Unphosphorylated STATs form an anti-parallel dimer/monomer equilibrium, and upon efficient recruitment to the cognate receptor–kinase complex, are phosphorylated on a specific tyrosine residue, which promotes parallel dimerization by conformational rearrangement. The activated STAT dimer translocates to the nucleus, initiating transcription of target genes and altering chromatin involved in loop formation in enhancer-promoter landscapes. The canonical domains of the STAT family are all present with the coiled-coil domain (CCD, S138-T331), DNA-binding domain (DBD, F332-V470), linker domain (H471-D591), and SH2 domain (Q592-P685). Archetypical STAT-type SH2 domains are comprised of an anti-parallel β-sheet created by three β-strands (conventionally labeled βB-βD) surrounded by three α-helices (αA, αB’, and αB), which are also observed in STAT5B.

In order to gain insight into the structural basis of the N642H mutation, as well as to validate modeling studies on the differences between STAT5A/B, we crystalized human STAT5B. With these domain boundaries, human STAT5B was crystallized and diffracted to 3.29 Å resolution. The overall architecture of human STAT5B is analogous to mouse STAT5A with a rmsd of 1.21 Å, and a rmsd of 1.89 Å and 2.03 Å, in comparison to mouse STAT3 and human STAT1 respectively. Within these domain boundaries, there are 29 amino acid differences between human STAT5B and mouse STAT5A, which are predominantly located within disordered regions and the SH2 domain. Conventional phospho-peptide binding occurs perpendicular to the central β-sheet with the phospho-Tyr accessing the N-terminal (pY) pocket on one face of the β-sheet and the flanking residues occupying the C-terminal (pY + 3) cavity on the opposite face. The pY-binding pocket is positively charged and harbors a number of evolutionarily conserved residues, such as an invariant arginine (R618 on βB5), that form part of the complex phosphate coordination network. The hydrophobic pY + 3 cavity serves as the peptide selectivity pocket and is predominantly formed by the βD strand and αB helix. As such, the surface-exposed βD strand controls access to both the phosphate-coordinating βB5 position and the selectivity residues located deeper in each of the N- and C- terminal pockets. Several of the variations between STAT5A and STAT5B occur within the βD strand and CD loop (Q636, M639, F640, M644), which ostensibly correlates to differences in peptide selectivity between the isoforms. The SH2 domain is a hot-spot for several mutations with the most prevalent mutations occurring either on the βD strand (such as N642H) or in close proximity ( < 5 Å apart), suggesting a common mechanism of action.

>[2x]STGSAMSQKHLQINQTFEELRLVTQDTENELKKLQQTQEYFIIQYQESLRIQAQFGPLAQLSPQERLSRETALQQKQVSLEAWLQREAQTLQQYRVELAEKHQKTLQLLRKQQTIILDDELIQWKRRQQLAGNGGPPEGSLDVLQSWCEKLAEIIWQNRQQIRRAEHLCQQLPIPGPVEEMLAEVNATITDIISALVTSTFIIEKQPPQVLKTQTKFAATVRLLVGGKLNVHMNPPQVKATIISEQQAKSLLKNENTRNDYSGEILNNCCVMEYHQATGTLSAHFRNMSLKRIKRSDRRGAESVTEEKFTILFESQFSVGGNELVFQVKTLSLPVVVIVHGSQDNNATATVLWDNAFAEPGRVPFAVPDKVLWPQLCEALNMKFKAEVQSNRGLTKENLVFLAQKLFNNSSSHLEDYSGLSVSWSQFNRENLPGRNYTFWQWFDGVMEVLKKHLKPHWNDGAILGFVNKQQAHDLLINKPDGTFLLRFSDSEIGGITIAWKFDSQERMFWNLMPFTTRDFSIRSLADRLGDLNYLIYVFPDRPKDEVYSKYYTPVPCESATAKAVDGYVKPQ> MPLDAGGQNSTQMVLAPGASIFRCRQCGQTISRRDWLLPMGGDHEHVVFNPAGMIF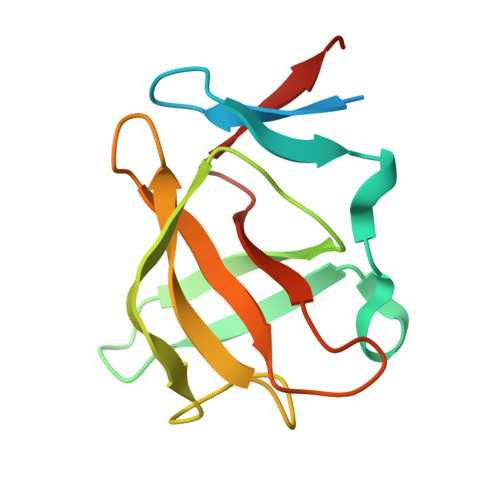RVWCFSLAQGLRLIGAPSGEFSWFKGYDWTIALCGQCGSHLGWHYEGGSQPQTFFGLIKDRLAEGPAD> MAINFKGSPYLDRFDPSKDRTKVLFNPDRPLQQAELNEMQSIDQYYLKNLGDAIFKDGDKQSGLGFTLSEDNVLTVNPGYVYINGKIRYYDNDDSVKITGVGKETIGIKLTERIVTPDEDASLLDQTSGVPSYFSKGADRLEEKMSLTVNDPTSATIYTFMDGDLYIQSTNAEMDKINKVLAERTYDESGSYKVNGFELFSEGNAEDDDHVSVVVDAGKAYVKGFKVDKPVSTRISVPKSYDLGTAENESTIFNKSNNSISLANSPVKEIRRVTGQVLIEKERVTRGAQGDGQDFLSNNTAFEIVKVWTETSPGVTTKEYKQGEDFRLTDGQTIDWSPQGQEPSGGTSYYVSYKYNKRMEAGKDYEVTTQGEGLSKKWYINFTPSNGAKPIDQTVVLVDYTYYLARKDSVFINKYGDIAILPGEPNIMRLVTPPLNTDPENLQLGTVTVLPDSDEAVCISFAITRLSMEDLQKVKTRVDNLEYNQAVNALDDGAMEGQNPLTLRSVFSEGFISLDKADITHPDFGIVFSFEDAEATLAYTEAVNQPKIIPGDTTAHIWGRLISAPFTEERTIYQGQASETLNVNPYNIPNKQGVLKLTPSEDNWIDTENVTITEQKTKKVTMKRFWRHNESYYGETEHYLYSNLQLDAGQKWKGETYAYDREHGRTGTLLESGGQRTLEEMIEFIRIRDVSFEVKGLNPNDNNLYLLFDGVRCAITPATGYRKGSEDGTIMTDAKGTAKGKFTIPAGIRCGNREVTLKNANSTSATTYTAQGRKKTAQDIIIRTRVTVNLVDPLAQSFQYDENRTISSLGLYFASKGDKQSNVVIQIRGMGDQGYPNKTIYAETVMNADDIKVSNNASAETRVYFDDPMMAEGGKEYAIVIITENSDYTMWVGTRTKPKIDKPNEVISGNPYLQGVLFSSSNASTWTPHQNSDLKFGIYTSKFNETATIEFEPIKDVSADRIVLMSTYLTPERTGCTWEMKLILDDMASSTTFDQLKWE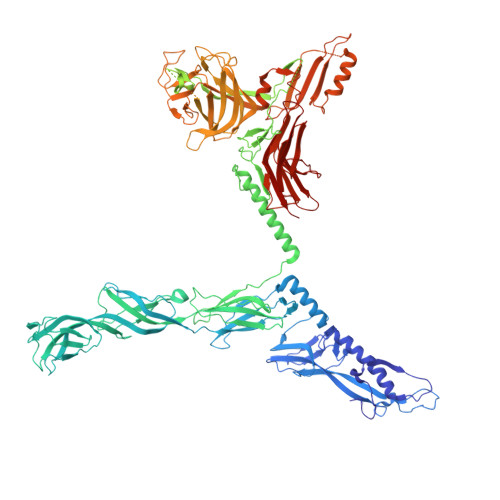PIGNYQDLDVLGLARQVKLRATFESNRYISPLMSSSDLTFTTFLTELTGSYVGRAIDMTEAPYNTVRFSYEAFLPKGTKVVPKYSADDGKTWKTFTKSPTTTRANNEFTRYVIDEKVKSSGTNTKLQVRLDLSTENSFLRPRVRRLMVTTRDE>[2x]MTSFAQLDIKSEELAIVKT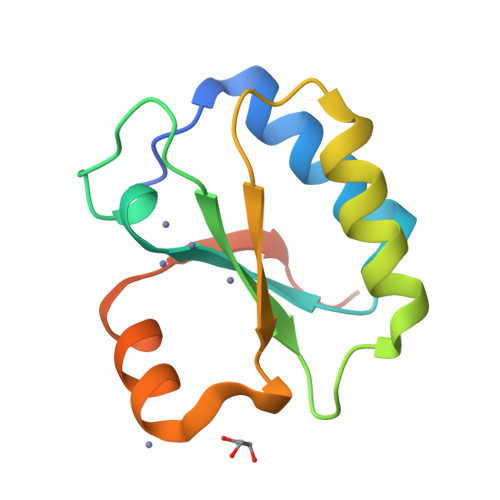ILQQLVPDYTVWAFGSRVKGKAKKYSDLDLAIISEEPLDFLARDRLKEAFSESDLPWRVDLLDWATTSEDFREIIRKVYVVIQEKEKTVEKPTAL>AHHHHHHSSGLEVLFQGPPEGAALTEKTDIFESGRNGNPNKDGIKSYRIPALLKTDKGTLIAGADERRLHSSDWGDIGMVIRRSEDNGKTWGDRVTITNLRDNPKASDPSIGSPVNIDMVLVQDPETKRIFSIYDMFPEGKGIFGMSSQKEEAYKKIDGKTYQILYREGEKGAYTIRENGTVYTPDGKATDYRVVVDPVKPAYSDKGDLYKGDQLLGNIYFTTNKTSPFRIAKDSYLWMSYSDDDGKTWSAPQDITPMVKADWMKFLGVGPGTGIVLRNGPHKGRILIPVYTTNNVSHLDGSQSSRVIYSDDHGKTWHAGEAVNDNRQVDGQKIHSSTMNNRRAQNTESTVVQLNNGDVKLFMRGLTGDLQVATSKDGGVTWEKDIKRYPQVKDVYVQMSAIHTMHEGKEYIILSNAGGPKRENGMVHLARVEENGELTWLKHNPIQKGEF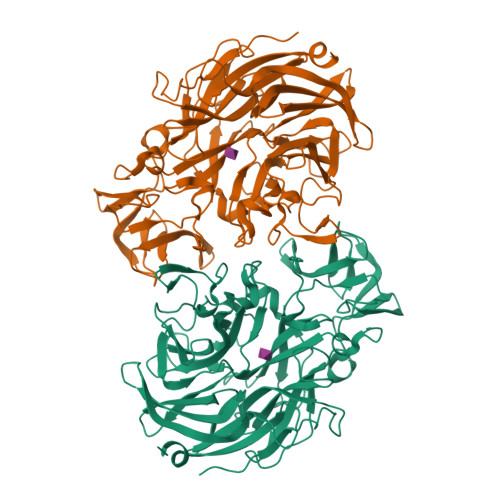AYNSLQELGNGEYGILYEHTEKGQNAYTLSFRKFNWEFLSKN[2x]> MFRM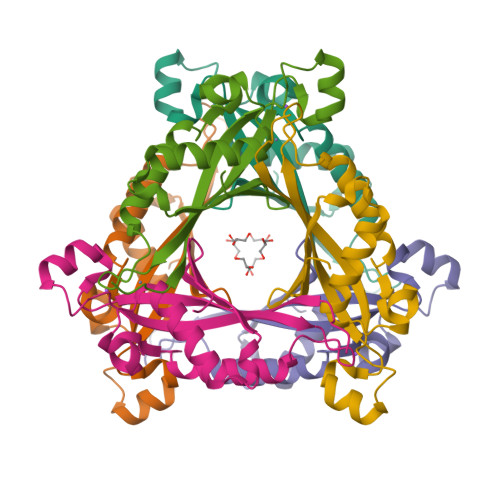PIVTMERVDSFSAAHRLHSEKLSDAENKETFGKCNNSNGHGHNYVWKVKLRGEVDPTSGMVYDLAKLKKEMSLVLDTVDHRNLDKDVEFFKTTVSTSENVAIYMFEKLKSVMSNPSVLYKVTIEETPKNIFTYKGS>[2x]GVSGSKGQKLFVSVLQRLLSERGLHVKESSAIEFYQFLIKVSPWFPEEGGLNLQDWKR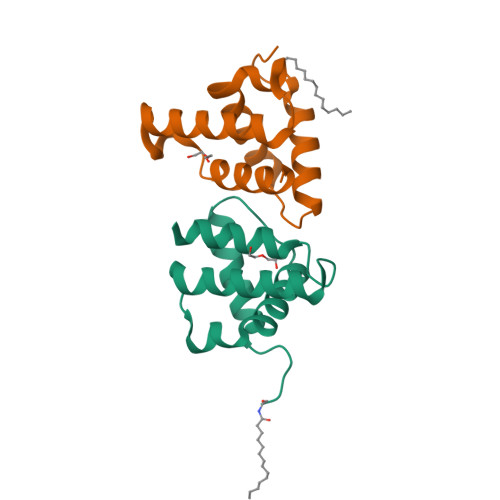VGREMKRYAAEHGTDSIPKQAAPIWLQLREILT> ASAKLPGDFGPPRGEPIHAVLTSPPLVPPPVNRTYPAKVIVELEVVEKEMQISEGVSYTFWTFGGTVPGSFIRVRQGDTVEFHLKNHPSSKMAHNIDLHGVTGPGGGAASSFTAPGHESQFTFKALNEGIYVYHCATAPVGMHIANGMYGLILVEPPEGLPKVDHEYYVMQGDFYTAGKYREKGLQPFDMEKAIDERPSYVLFNGAEGALTGDKALHAKVGETVRIFVGNGGPNLVSSFHVIGAIFDQVRYEGGTNVQKNVQTTLIPAGGAAVVKFTARVPGSYVLVDHSIFRAFNKGAMAILKIDGAENKLVYSGKELDSVYLGDRAAPNMSAVTKATQASVSGTLTVQDQVQAGRALFAGTCSVCHQGNGAGLPGVFP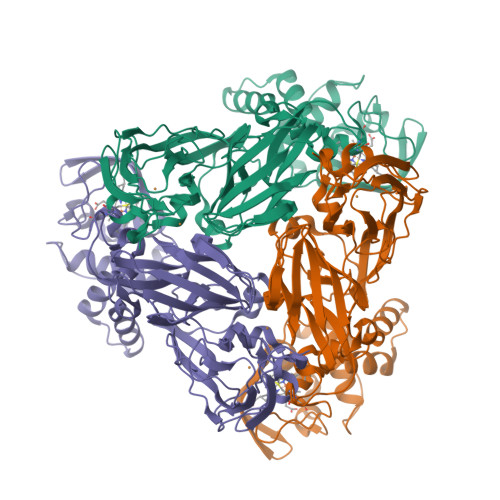PLAKSDFLAADPKRAMNIVLHGLNGKIKVNGQEYDSVMPPMTQLNDDEVANILTYVLNSWDNPGGRVSAEDVKKVRAQPAPAKAVAEH>GAMGRRLGVMGGTFDPIHYGHLVAASEVADLFDLDEVVFVPSGQPWQKGRQVSAAEHRYLMTVIATASNPRFSVSRVDIDRGGPTYTKDTLADLHALHPDSELYFTTGADALASIMSWQGWEELFELARFVGVSRPGYELRNEHITSLLGQLAKDALTLVEIPALAISSTDCRQRAEQSRPLWYLMPDGVVQYVS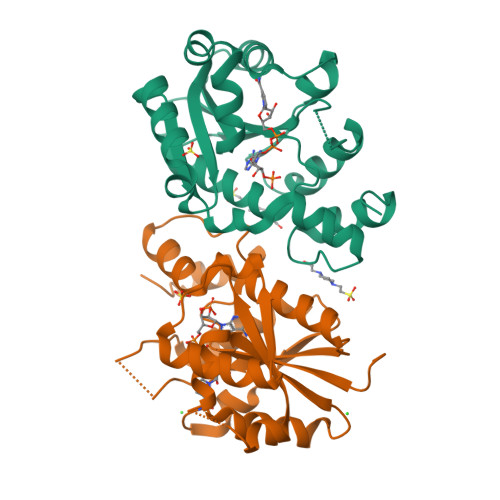KRRLYT[2x]>MGSDSIDTPNYDVQKHINKLCGMLLITEDANHKFTGLIGMLYAMSRLGREDTIKILRDAGYHVKANGVDVTTHRQDINGKEMKFEVLTLASLTTEIQINIEIESRKSYKKMLKEMGEVAPEYRHDSPDCGMIILCIAALVITKLAAGDRSGLTAVIRRANNVLKNEMKRYKGLLPKDIANSFYEVFEKHPHFI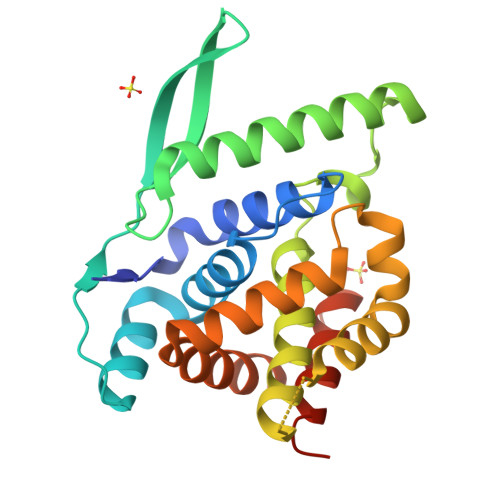DVFVHFGIAQSSTRGGSRVEGIFAGLFMNAYGLEHHHHHH[2x];> EDF> SEQNNAVLPKGVTQGEFNKAVQKFRALLGDDNVLVESDQLVPYNKIMMPVENAAHAPSAAVTATTVEQVQGVVKICNEHKIPIWTISTGRNFGYGSAAPVQRGQVILDLKKMNKIIKIDPEMCYALVEPGVTFGQMYDYIQENNLPVMLSFSAPSAIAGPVGNTMDRGVGYTPYGEHFMMQCGMEVVLANGDVYRTGMGGVPGSNTWQIFKWGYGPTLDGMFTQANYGICTKMGFWLMP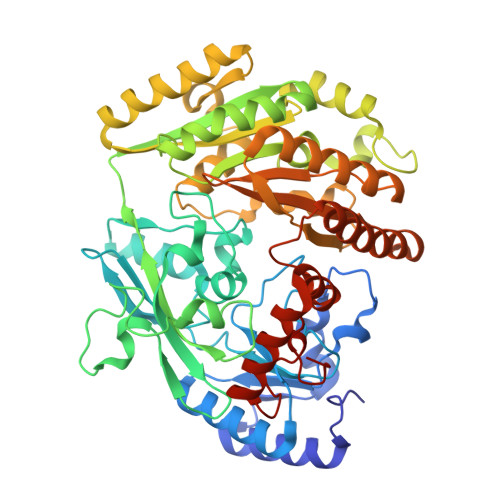KPPVFKPFEVIFEDEADIVEIVDALRPLRMSNTIPNSVVIASTLWEAGSAHLTRAQYTTEPGHTPDSVIKQMQKDTGMGAWNLYAALYGTQEQVDVNWKIVTDVFKKLGKGRIVTQEEAGDTQPFKYRAQLMSGVPNLQEFGLYNWRGGGGSMWFAPVSEARGSECKKQAAMAKRVLHKYGLDYVAEFIVAPRDMHHVIDVLYDRTNPEETKRADACFNELLDEFEKEGYAVYRVNTRFQDRVAQSYGPVKRKLEHAIKRAVDPNNILAPGRSGIDLNNDF>[2x]MEEECRVLSIQSHVIRGYVGNRAATFPLQVLGFEIDAVNSVQFSNHTGYAHWKGQVLNSDELQELYEGLRLNNMNKYDYVLTGYTRDKSFLAMVVDIVQELKQQNPRLVYV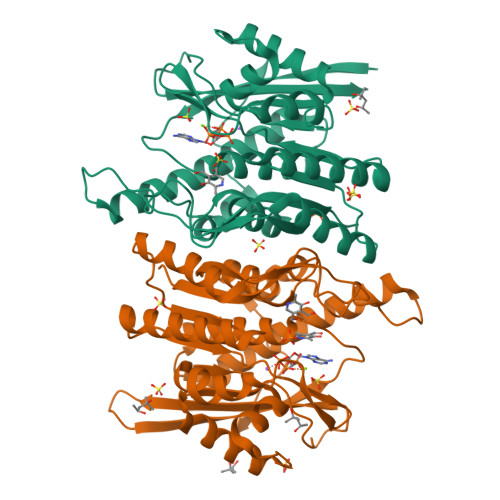CDPVLGDKWDGEGSMYVPEDLLPVYKEKVVPLADIITPNQFEAELLSGRKIHSQEEALRVMDMLHSMGPDTVVITSSDLPSPQGSNYLIVLGSQRRRNPAGSVVMERIRMDIRKVDAVFVGTGALFAAMLLAWTHKHPNNLKVACEKTVSTLHHVLQRTIQCAKAQAGEGVRPSPMQLELRMVQSKRDIEDPEIVVQATVL> MEEKEILWNEAKAFIAACYQELGKAAEVKDRLADIKSEIDLTGSYVHTKEELEHGAKMAWRNSNRCIGRLFWNSL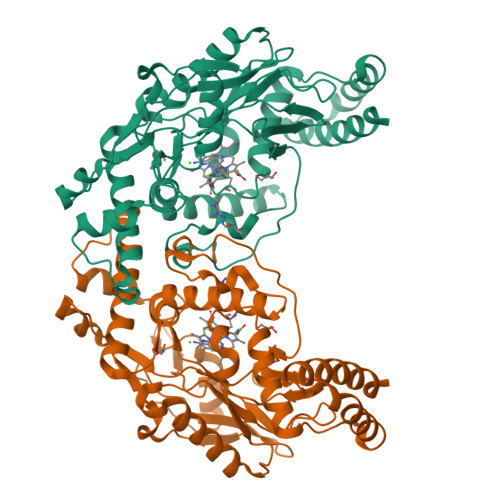NVIDRRDVRTKEEVRDALFHHIETATNNGKIRPTITIFPPEEKGEKQVEIWNHQLIRYAGYESDGERIGDPASCSLTAACEELGWRGERTDFDLLPLIFRMKGDEQPVWYELPRSLVIEVPITHPDIEAFSDLELKWYGVPIVSDMKLEVGGIHYNAAPFNGWYMGTEIGARNLADEKRYDKLKKVASVIGIAADYNTDLWKDQALVELNKAVLHSYKKQGVSIVDHHTAASQFKRFEEQAEEAGRKLTGDWTWLIPPISPAATHIFHRSYDNSIVKPNYFYQDKPYE> MYYGISQFSEAYNKILRNSSSHSSCQLVIFVSCLNIDALCATKMLSLLFKKQLVQSQIVPIFGYSELRRHYSQLDDNINSLLLVGFGGVIDLEAFLEIDPQEYVIDTDEKSGEQSFRRDIYVLDAHRPWNLDNIFGSQIIQCFDDGTVDDTLGEQKEAYYKLLELDEESGDDELSGDENDNNGGDDEATDADEVTDEDEEDEDETISNKRGNSSIGPNDLSKRKQRKKQIHEYEGVLEEYYSQGTTVVNSISAQIYSLLSAIGETNLSNLWLNILGTTSLDIAYAQVYNRLYPLLQDEVKRLTPSSRNSVKTPDTLTLNIQPDYYLFLLRHSSLYDSFYYSNYVNAKLSLWNENGKKRLHKMFARMGIPLSTAQETWLYMDHSIKRELGIIFDKNLDRYGLQDIIRDGFVRTLGYRGSISASEFVEALTALL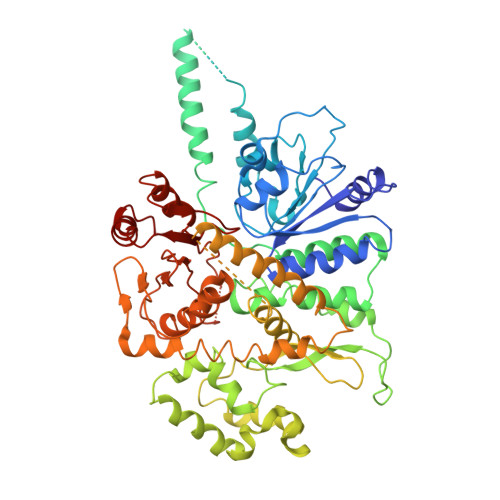EVGNSTDKDSVKINNDNNDDTDGEEEEDNSAQKLTNLRKRWVSNFWLSWDALDDRKVELLNRGIQLAQDLQRAIFNTGVAILEKKLIKHLRIYRLCVLQDGPDLDLYRNPLTLLRLGNWLIECCAESEDKQLLPMVLASIDENTDTYLVAGLTPRYPRGLDTIHTKKPILNNFSMAFQQITAETDAKVRIDNFESSIIEIRREDLSPFLEKLTLSGLL>[8x]GPLGSNRRLQQTQAQVDEVVDIMRVNVDKVLER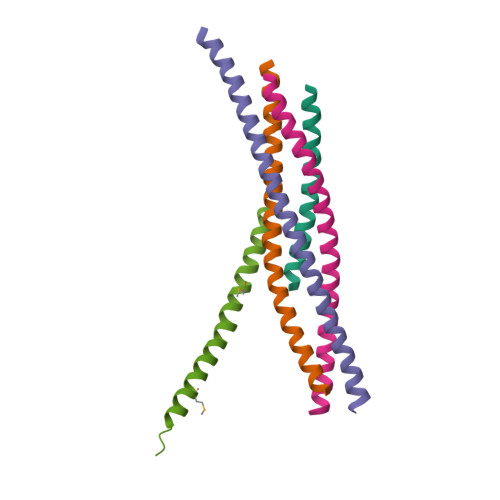DQKL;>GSALSEIETRHSEIIKLENSIRELHDMFMDMAMLVESQGEMIDRIEYNVEHAVDYVERAVSDTKK[8x];>[8x]GSHMMRNELEEMQRRADQLADESLESTRRMLQLVEESKDAGIRTLVMLDEQGEQLDRVEEGMNHINQDMKEAEKNLKDLGW;>[8x]GSARENEMDENLEQVSGIIGNLRHMALDMGNEIDTQNRQIDRIMEKADSNKTRIDEANQRATKML;>GPLGSKLPDAAKKMEEAQEALRQAEEERKAKYAKMEAEREAVRQGIRDKYGIKKKEEREAEAQ[8x]> MAKKKTVPAMDFFASLERVSDAEDKNVNLDVGKELPEQLKDDEDGKVNPCDEVTNVVTNTPIDVCKGPDVDGTADKINDKKIHVSQGLKEFQVAKGDRVENEITETADEMITKVSDTKDLNVSTKKPHQIADVPSNEDISIMEANETEQLDHGYDATALLETTEDIITGELDDHLESLSVEMFTIVNELTKVESVQTALENYIGLVSNRHHRGHDVDHDLAKAISIALESFDYKYFNNTVPSMESFISPLTRPKASIEVLDNLQAKAKEVSTVALDFIKKLIRIVVETYQRIRQNVSNQIERVNKIMKRVKENELPDEVRTIAIPRDLILGDTGESWVGVDPVQGVTVIRNLFDSIEKNGLRALKAALAGKTTDDKALALAKGMFGTATKINANGVRYASPVVPGNRVYTFGKDKAAVDFSILDAPGKPNYGITVELLVDKNVVMAQLKAVHN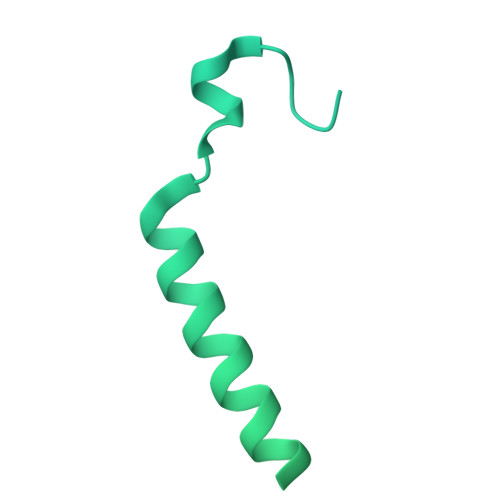LLNHLNNIRGISKESTAEIIAQMTDKEATNVGKAYLTGTTEASNDLFKCVMIWITVLEKLVDSEIKETE>LEVQNSCDNCQPGTFCRKYNPVCKSCPPSTFSSIGGQPNCNICRVCAGYFRFKKFCSSTHNAECECIEGFHCLGPQCTRCEKDCRPGQELTKQGCKTCSLGTFNDQNGTGVC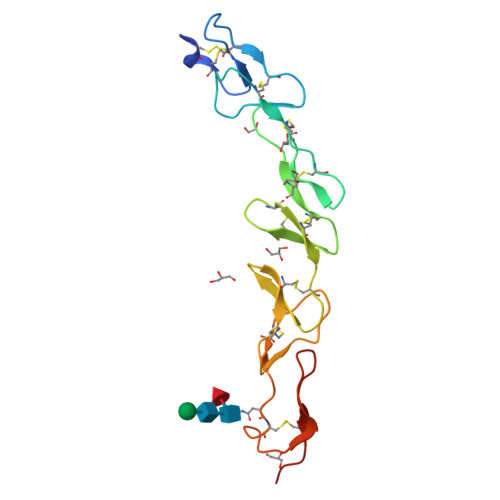RPWTNCSLDGRSVLKTGTTEKDVVCGPLVPR[4x]>[4x]SGIVPTLQNIVATVTLGCRLDLKTVALHARNA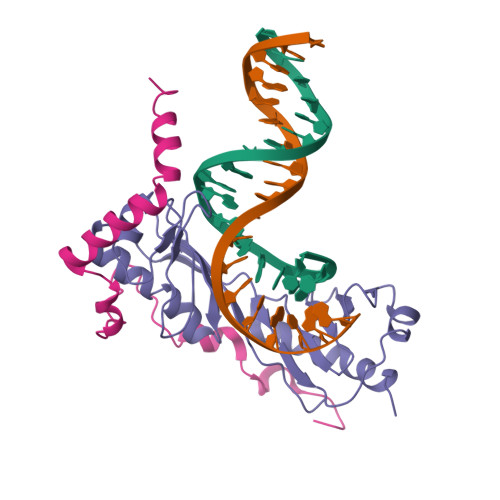EYNPKRFAAVIMRIREPKTTALIFASGKMVVTGAKSEDDSKLASRKYARIIQKIGFAAKFTDFKIQNIVGSCDVKFPIRLEGLAFSHGTFSSYEPELFPGLIYRMVKPKIVLLIFVSGKIVLTGAKQREEIYQAFEAIYPVLSEFRKM;>[4x]GSYCPRNLHLLPTTDTYLSKVSDDPDNLEDVDDEELNAHLLNEEASKLKERIWIGLNADFLLEQESKRLKQE> PLLYSTDDAICSKANELLQRSRQVQNKTEKERMLRESLKEYQKISNQVDLSNVCAQYRQVR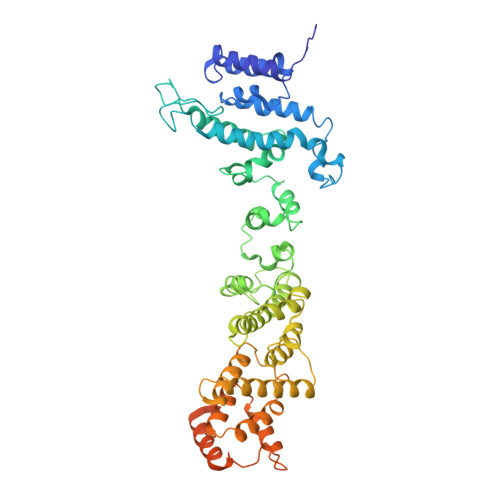FYEGVVELSLTAAEKKDPQGLGLHFYKHGEPEEDIVGLQAFQERLNSYKCITDTLQELVNQSKAAPQSPSVPKKPGPPVLSSDPNMLSNEEAGHHFEQMLKLSQRSKDELFSIALYNWLIQVDLADKLLQVASPFLEPHLVRMAKVDQNRVRYMDLLWRYYEKNRSFSNAARVLSRLADMHSTEISLQQRLEYIARAILSAKSSTAISSIAADGEFLHELEEKMEVARIQLQIQETLQRQYSHHSSVQDAVSQLDSELMDITKLYGEFADPFKLAECKLAIIHCAGYSDPILVQTLWQDIIEKELSDSVTLSSSDRMHALSLKIVLLGKIYAGTPRFFPLDFIVQFLEQQVCTLNWDVGFVIQTMNEIGVPLPRLLEVYDQLFKSRDPFWNRMKKPLHLLDCIHVLLIRYVENPSQVLNCERRRFTNLCLDAVCGYLVELQSMSSSVAVQAITGNFKSLQAKLERLH CRISPR-Cas are adaptive immune systems in bacteria and archaea that utilize CRISPR RNA-guided surveillance complexes to target complementary RNA or DNA for destruction. Recently, a variant type III-D system (III-Dv) was annotated with multiple gene fusions, suggesting its role as an evolutionary intermediate between the multi- and single-subunit type III effectors. The operon of the type III-Dv complex from Synechocystis sp. PCC6803 contains cas10, a cas7-cas5-cas11 fusion, a double cas7 fusion (cas7-2x), csx19, and an insertion-containing cas7 (cas7-insertion). Here, we present cryo-electron microscopy (cryo-EM) structures of the type III-Dv complex in four distinct states: bound to a crRNA (binary, surveillance complex), bound to an RNA non-self target in a pre-cleavage state, and bound to a self-target with coordinated magnesium in pre-cleavage and post-cleavage states.

We determined the cryo-EM structure of the type III-Dv surveillance complex containing the 37-nt crRNA at a global resolution of 2.5 Å, enabling us to fit and refine AlphaFold2-predicted models and rapidly generate a complete atomic model for the complex. Native mass-spectrometry revealed that a single copy of each subunit assembled into a 332 kDa complex, in contrast to type III-A and -B complexes which contain multiple copies of Cas7 and Cas11 subunits. Despite the different subunit stoichiometries compared with other type III complexes, our structure revealed that the fused subunits still arrange into a repeating backbone around the crRNA, a structural feature conserved across all class 1 CRISPR-Cas complexes. An uncharacterized domain comprising the N-terminal 112 residues of the Cas7-insertion subunit was absent from our map, likely due to flexibility. Csx19, a subunit unique to type III-D1 and III-Dv, contains multiple β-sheets and is nestled at the base of the effector between Cas5 and Cas10 subunits, making contacts with the crRNA, and contributing to the structural integrity of the complex. Indeed, affinity purification of a ΔCsx19 complex with an N-terminal Cas10 tag did not result in pulldown of the complex, indicating that assembly of Csx19 onto the type III-Dv complex is essential for complex assembly and stability. Our structure supports this evolutionary relationship, as the organization of the type III-D1 operon is maintained and subunits are physically fused together through flexible ~20-residue linker polypeptides. This is exemplified by the Cas7-Cas5-Cas11 subunit, which adopts a tortuous topology that places Cas7 in the body of the complex, Cas5 below it, and Cas11 back on top of Cas7. While most of the crRNA spacer is completely buried within the type III-Dv complex, six bases at the 3′ end are highly exposed in the insertion domain of the Cas7-insertion subunit.

> MRGIEITITMQSDWHVGTGMGRGELDSVVQRDGDNLPYIPGKTLTGILRDSCEQVALGLDNGQTRGLWHGWINFIFGDQPALAQGAIEPEPRPALIAIGSAHLDPKLKAAFQGKKQLQEAIAFMKPGVAIDAITGTAKKDFLRFEEVVRLGAKLTAEVELNLPDNLSETNKKVIAGILASGAKLTERLGGKRRRGNGRCELKFSGYSDQQIQWLKDNYQSVDQPPKYQQNKLQSAGDNPEQQPPWHIIPLTIKTLSPVVLPARTVGNVVECLDYIPGRYLLGYIHKTLGEYFDVSQAIAAGDLIITNATIKIDGKAGRATPFCLFGEKLDGGLGKGKGVYNRFQESEPDGIQLKGERGGYVGQFEQEQRNLPNTGKINSELFTHNTIQDDVQRPTSDVGGVYSYEAIIAGQTFVAELRLPDSLVKQITSKNKNWQAQLKATIRIGQSKKDQYGKIEVTSGNSADLPKPTGNNKTLSIWFLSDILLRGDRLNFNATPDDLKKYLENALDIKLKERSDNDLICIALRSQRTESWQVRWGLPRPSLVGWQAGSCLIYDIESGTVNAEKLQELMITGIGDRCTEGYGQIGFNDPLLSASLGKLTAKPKASNNQSQNSQSNPLPTNHPTQDYARLIEKAAWREAIQNKALALASSRAKREEILGIKIMGKDSQPTMTQLGGFRSVLKRLHSRNNRDIVTGYLTALEQVSNRKEKWSNTSQGLTKIRNLVTQENLIWNHLDIDFSPLTITQNGVNQLKSELWAEAVRTLVDAIIRGHKRDLEKAQENESNQQSQGAA;> MPAGGRLMKNLYHYHQYEITLESAVDSCKNHLQAAIGLLYSPQKCELVKLDNSGKLVDSYNRLKFNNLGVFEARFFNLNCELRWVNESNGNGTAVLLSESDITLTGFEKGLQEFITAIDQQYLLWGEPAKHPPNADGWQRLAEARIGKLDIPLDNPLKPKDRVFLTSEEYIAEVDDFGNCAVIDERLIKLEVK;> MAHHHHHHVGTENLYFQGFLVLIETSGNQHFIFSTNKLRENIGASELTYLATTEILFQGVDRVFQTNYYDQWSDTNSLNFLADSKLNPAIDDPKNNADIEILLATSGKAIALVKEEGKAKQLIKEVTKQALINAPGLEIGGIYVNCNWQDKLGVAKAVKEAHKQFEVNRAKRAGANGRFLRLPIAAGCSVSELPASDFDYNADGDKIPVSTVSKVKRETAKSAKKRLRSVDGRLVNDLAQLEKSFDELDWLAVVHADGNGLGQILLSLEKYIGEQTNRNYIDKYRRLSLALDNCTINAFKMAIAVFKEDSKKIDLPIVPLILGGDDLTVICRGDYALEFTREFLEAFEGQTETHDDIKVIAQKAFGVDRLSACAGISIIKPHFPFSVAYTLAERLIKSAKEVKQKVTVTNSSPITPFPCSAIDFHILYDSSGIDFDRIREKLRPEDNTELYNRPYVVTAAENLSQAQGYEWSQAHSLQTLADRVSYLRSEDGEGKSALPSSQSHALRTALYLEKNEADAQYSLISQRYKILKNFAEDGENKSLFHLENGKYVTRFLDALDAKDFFANANHKNQGE;> MARKVTTRWKITGTLIAETPLHIGGVGGDADTDLALAVNGAGEYYVPGTSLAGALRGWMTQLLNNDESQIKDLWGDHLDAKRGASFVIVDDAVIHIPNNADVEIREGVGIDRHFGTAANGFKYSRAVIPKGSKFKLPLTFDSQDDGLPNALIQLLCALEAGDIRLGAAKTRGLGRIKLDDLKLKSFALDKPEGIFSALLDQGKKLDWNQLKANVTYQSPPYLGISITWNPKDPVMVKAEGDGLAIDILPLVSQVGSDVRFVIPGSSIKGILRTQAERIIRTICQSNGSEKNFLEQLRINLVNELFGSASLSQKQNGKDIDLGKIGALAVNDCFSSLSMTPDQWKAVENATEMTGNLQPALKQATGYPNNISQAYKVLQPAMHVAVDRWTGGAAEGMLYSVLEPIGVTWEPIQVHLDIARLKNYYHGKEEKLKPAIALLLLVLRDLANKKIPVGYGTNRGMGTITVSQITLNGKALPTELEPLNKTMTCPNLTDLDEAFRQDLSTAWKEWIADPIDLCQQEAA;> MTVGTLGVVGSAKNLKLQLSFINTRQQYVQITLFERNSFKVAEEEFSTELVEIIKTALPTLKNKKVEFEEDGDQIKQIREKGQAWVGAAEQIAPYVLPSGNITETPRNVNASNFHNPYNFVPALPRDGITGDLGDCAPAGHSYYHGDKYSGRIAVKLTTVTPLLIPDASKEEINNNHKTYPVRIGKDGKPYLPPTSIKGMLRSAYEAVTNSRLAVFEDHDSRLAYRMPATMGLQMVPARIEGDNIVLYPGTSRIGNNGRPANNDPMYAAWLPYYQNRIAYDGSRDYQMAEHGDHVRFWAERYTRGNFCYWRVRQIARHNQNLGNRPERGRNYGQHHSTGVIEQFEGFVYKTNKNIGNKHDERVFIIDRESIEIPLSRDLRRKWRELITSYQEIHKKEVDRGDTGPSAVNGAVWSRQIIADESERNLSDGTLCYAHVKKEDGQYKILNLYPVMITRGLYEIAPVDLLDETLKPATDKKQLSPADRVFGWVNQRGNGCYKGQLRIHSVTCQHDDAIDDFGNQNFSVPLAILGQPKPEQARFYCADDRKGIPLEDGYDRDDGYSDSEQGLRGRKVYPHHKGLPNGYWSNPTEDRSQQAIQGHYQEYRRPKKDGLEQRDDQNRSVKGWVKPLTEFTFEIDVTNLSEVELGALLWLLTLPDLHFHRLGGGKPLGFGSVRLDIDPDKTDLRNGAGWRDYYGSLLETSQPDFTTLISQWINAFQTAVKEEYGSSSFDQVTFIKASGQSLQGFHDNASIHYPRSTPEPKPDGEAFKWFVANEKGRRLALPALEKSQSFPIKPS> MGSSHHHHHHSQDPFSECNDEIDNAKLIMKERRFTASYTFAKFSTGSMLLTKDIVGKSGVSIKRLPTELQRKFLFDDVYLDKEIEKVTIEARKSNPYPQISESSLLFKDALDYMEKTSSDYNLWKLSSILFDPVSYPYKTDNDQVKMALLKKERHCRLTSWIVSQIGPEIEEKIRNSSNEIEQIFLYLLLNDVVRASKLAIE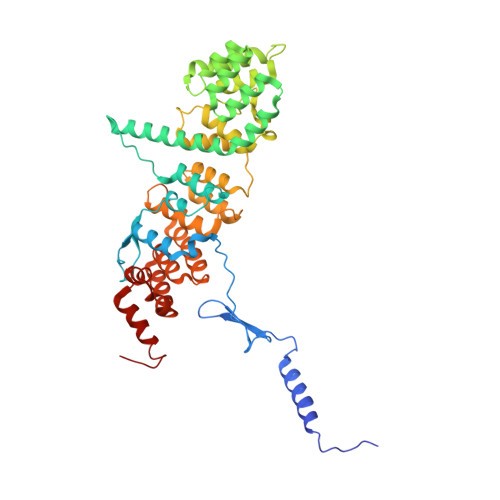SKNGHLSVLISYLGSNDPRIRDLAELQLQKWSTGGCSIDKNISKIYKLLSGSPFEGLFSLKELESEFSWLCLLNLTLCYGQIDEYSLESLVQSHLDKFSLPYDDPIGVIFQLYAANENTEKLYKEVRQRTNALDVQFCWYLIQTLRFNGTRVFSKETSDEATFAFAAQLEFAQLHGHSLFVSCFLNDDKAAEDTIKRLVMREITLLRASTNDHILNRLKIPSQLIFNAQALKDRYEGNYL> VDKNYTVSAKDSAKLIEEVRKALEVKFEDTKAGANVNDRVYDIKVDNVNLTNATQLQNKINSLTEGQSLKVTIQDKGHQVLGGKVVDYKIENYKTAQEIVDAVNAYNATLAEDSDNKLTATIKSTNTVEVKRAKDSANVITLNVGDQHLDFSKVITSEEGTFEGYEKRYSDIDSKELHTVTVKNADLQDISAEELFDGIRLTTLGREIVNKVKNGYALTFENEAILTQEQEDSDDKDKPEKSSFDIVLSKANEKPETISVSSKNHKLVRDLHKVLTDVKDGKELKVEVLSGDSRFTTAVEVSKERFKDGEAEAIILVGEDAIVDGLASAPLASQKNAPILLSKKDSLPSEIEAEILRVLGSNLSSKKIYIVGGESKVSKETEEKLSKLGVSKVERVSGEDRFETSLEIAKQLKDTFKTAFVVGGNGEADAMSISARAAQFGAPIIVTGNELDANAEKLLKGKELEIVGGENS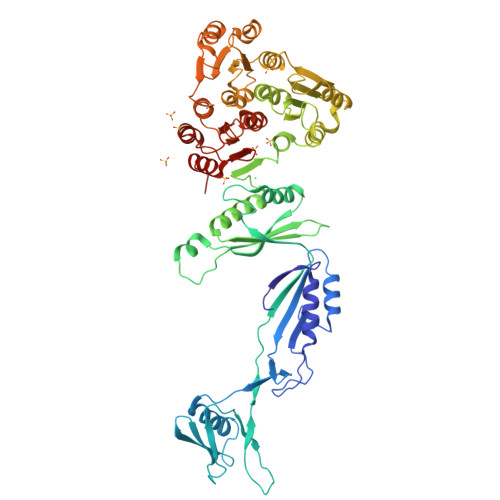VSKEVEDKLVDIDLNNKVERLAGENRKDTNAKVINKYYAGATKAYVAKDGYVGGNGQLVDALTAAPLAASSKAPIVLTTEELSKSQEEVVELRLKNATKLVQIGEGIAKNAIEKIAEKINLFT> QHQHQHQHQHQQPNEEFRPEMLQGKKVIVTGASKGIGREMAYHLAKMGAHVVVTARSKETLQKVVSHCLELGAASAHYIAGTMEDMTFAEQFVAQAGKLMGGLDMLILNHITNTSLNLFHDDIHHVRKSMEVNFLSYVVLTVAALPMLKQ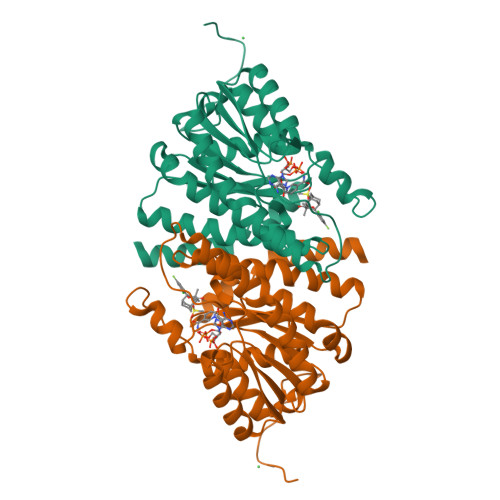SNGSIVVVSSLAGKVAYPMVAAYSASKFALDGFFSSIRKEYSVSRVNVSITLCVLGLIDTETAMKAVSGIVHMQAAPKEECALEIIKGGALRQEEVYYDSSLWTTLLIRNPSRKILEFLYSTSYN> MPPQLHNGLDFSAKVIQGSLDSLPQEVRKFVEGNAQLCQPEYIHICDGSEEEYGRLLAHMQEEGVIRKLKKYDNCWLALTDPRDVARIESKTVIITQEQRDTVPIPKSGQSQLGRWMSEEDFEKAFNARFPGCMKGRTMYVIPFSMGPLGSPLAKIGIELTDSPYVVASMRIMTRMGTSVLEALGDGEFIKCLHSVGCPLPLKKPLVNNWACNPELTLIAHLPDRREIISFGSGYGGNSLLGKKCFALRIASRLAKEEGWLAEHMLILGITNPEGKKKYLAAAFPSACGKTNLAMMNPTLPGWKVECVGDDIAWMKFDAQGNLRAINPENGFFGVAPGTSVKTNPNAIKTIQKNTIFTNVAETSDGGVYWEGIDEPLAPGVTITSWKNKEWRPQDEEPC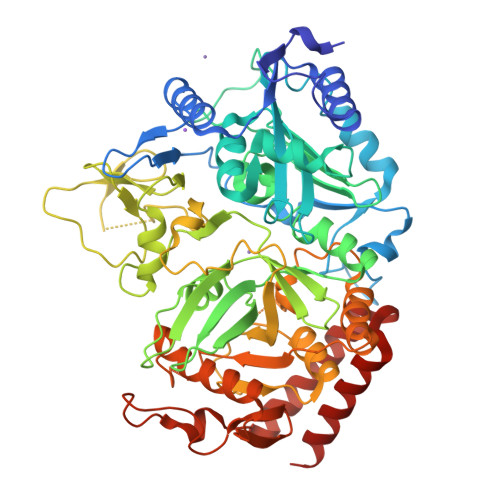AHPNSRFCTPASQCPIIDPAWESPEGVPIEGIIFGGRRPAGVPLVYEALSWQHGVFVGAAMRSEATAAAEHKGKVIMRDPFAMRPFFGYNFGKYLAHWLSMAHRPAAKLPKIFHVNWFRKDKNGKFLWPGFGENSRVLEWMFGRIEGEDSAKLTPIGYVPKEDALNLKGLGDVNVEELFGISKEFWEKEVEEIDKYLEDQVNADLPYEIERELRALKQRISQM> MNYKKVEASDIAAIKELIPAERVFVGTEIGEDFSHDELGSIHSYPEVLIKVTSTEEVSKIMKYAYEHNIPVVVRGSGTGLVGACVPLFGGIMLETTLMNNILELDTENLTVTVEPGVLLMELSKFVEENDLFYPPDPGEKSATIAGNISTNAGGMRAVKYGVTRDYVRGLTVVLANGEIIELGGKIVKNSSGYSLKDLVIGSEGTLCVITKAILKLLPLPKMTLSLLIPFENISDAAGIVPKIIKSKAIPTAIEFMERQTILFAEDFLGKKFPDSSSNAYILLTFDGNTKEQVEAEYETVANLCLAEGAKDVYIVDTVERKDSVWSARGAFLEAIKASTTEMDECDVVVPRNRIAEFIEFTHDLAKEMDVRIPSFGHAGDGNLHIYVCRDELCQADWEAKLAEAMDRMYAKALTFEGLVSGEHGIGYAKRKYLLNDFGTEHLALMAGIKQTF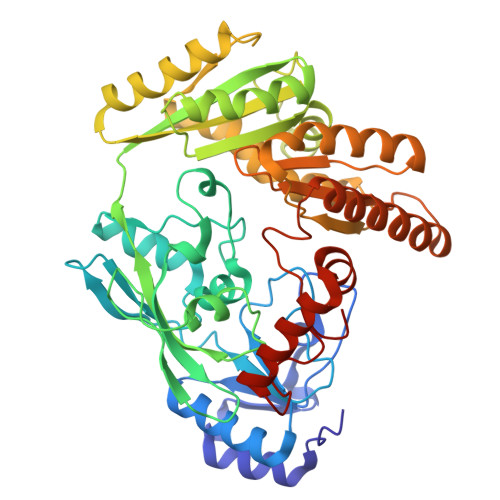DPKNLLNPKKVCQMA> GPLGSMDPDTFSDNFNNRPIASRRNTVYLCYEVKTKGPSRDAKIFRGQAASEDKYHPEMRFLSLVSKWRDQEYEVTWYISWSPCTKCARDMATFLQENTHVTLTIFVARLYAAADPDYQEALRSLAQAGATIKIMNYDEFQHCWSKFVYSQGAPFQPWDGLDEHSQALSGRLGEILRHSMDAATFTFNFNNEP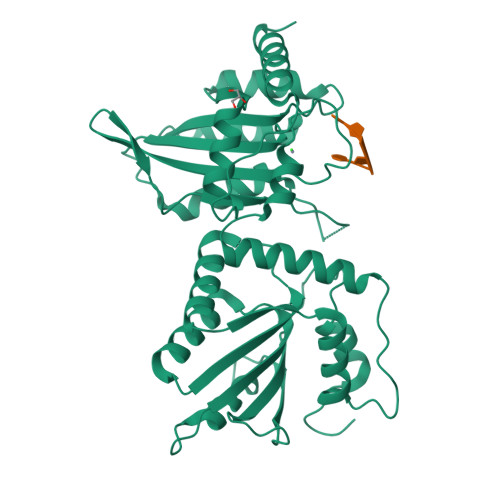WVRGRHETYLCYEVERMHNDTWVKLAQRRGFLANQAKHKHGFLEGRHAALCFLDVIPFWKLDLDQDYRVTCFTSWSPCFSCAQEMAKFISKNKHVSLCIKTARIYDDKGRAAEGLRTLAEAGAKISIMTYSEFKHCWDTFVDHQGAPFQPWDGLDEHSQDLSGRLRAILQNQEN> XMEMLTKFESRSSRAKGVAFHPTQPWILTSLHNGRIQLWDYRMGTLLDRFDGHDGPVAGIAFHPTQPLFVSGGDDYKVNVWNYKS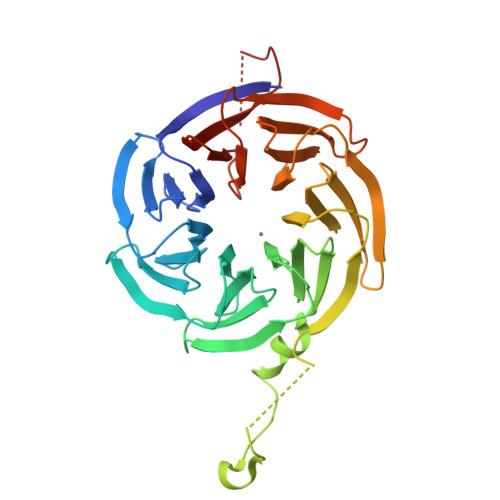RKLLFSLCGHMDYVRVCTFHHEYPWILSCSDDQTIRIWNWQSRNCIAILTGHSHYVMCAAFHPSEDLIVSASLDQTVRVWDISGLRMKNAAPVSMSKEDQKAQAHNSKSNDKKGSTDAIVKFVLEGHDRGVNWCAFHPTLPLILSAGDDRLVKLWRMTASKAWEVDTCRGHFNNVSCCLFHPHQELILSASEDKTIRVWDLNRRTAVQTFRRDNDRFWFITVHPKLNLFAAAHDSGVMVFKLESAWSHPQFEK>[4x]SHMSNKEYRPTLAQLRTFVTIAECKHFGTAATKLSISQPSLSQALVALETGLGVQLIERSTRKVIVTPAGEKLLPFAKSTLDAAESFLSHAKGANGSLTGPLTVGIIPTAAPYILPSMLSIVDEEYPDLEPHIVEDQTKHLLALLRDGAIDVAMMALPSEAPGMKEIPLYDEDFIVVTASDHPFAGRQDLELSALEDLDLLLLDDGH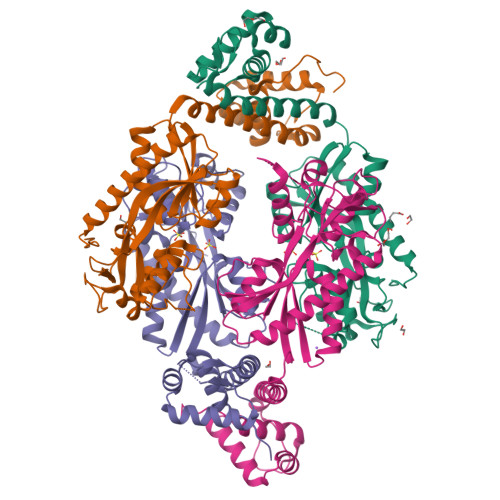SLHDQIVDLCRRGDINPISSTTAVTRASSLTTVMQLVVAGLGSTLVPISAIPWECTRPGLATANFNSDVTANRRIGLVYRSSSSRAEEFEQFALILQRAFQEAVALAASTGITLKQNVAVAQ2-amino-5-[3-(1-ethyl-1H-pyrazol-5-yl)-1H-pyrrolo[2,3-b]pyridin-5-yl]-N,N-dimethylbenzamide | C21 H22 N6 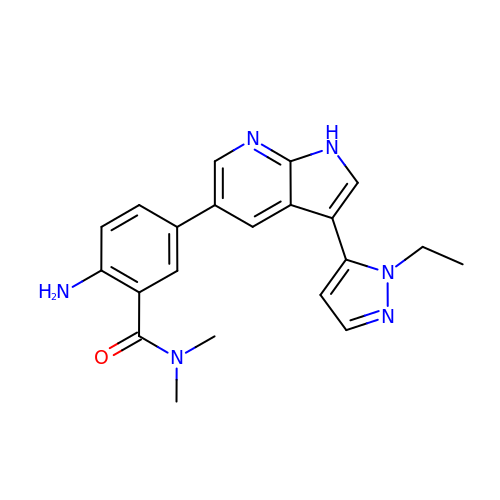O | INAGORZAOFUKOZ-UHFFFAOYSA-N Ribonuclease E (RNase E) is a metal-dependent hydrolytic enzyme that cleaves polymeric ribonucleic acid internally and serves as a central element in RNA metabolism of diverse bacteria. The NTD of RNase E (1–529) is highly conserved and harbors the catalytic activity of the enzyme. RNase E forms a tetramer in which the protomers are arranged as a dimer of dimers and accommodate an RNA substrate at the active site formed by the interface of two subunits of the principal dimer unit. The catalytic site is located in a DNase I-like domain, where conserved acidic groups D303 and D346 coordinate the magnesium ions that assist in the hydrolytic attack of single-stranded RNA.

In an effort to structurally characterize the mechanism of 5′ end sensing by RNase E and its interaction with sRNA, the catalytically inactive RNase E (1–529) D303R, D346R was purified and used in co-crystallization trials with sRNA bearing a 5′ monophosphate. The oligoribonucleotide comprises the MicC seed region connected through a tetranucleotide loop with a fragment of the ompD target encompassing the seed complementary sequence and the RNase E cleavage site (Pfeiffer et al., 2009). Crystals of the protein:RNA complex were obtained, and an X-ray diffraction dataset was collected to 3.0 Å resolution. An RNA fragment of 2 to 3 bases could be modeled with a good fit to the density at each of the two independent 5′ sensor domains in the crystallographic asymmetric unit. Given that the 5′ sensor domain is known to bind the 5′ end of RNA substrates, the RNA density was modeled as the 5′ end of MicC. The 5′ monophosphate is bound in the 5′ sensing pocket, and the RNA forms additional contacts with RNase E that were not seen in the previous structure of the “closed” state, where the substrate is bound at the active site. For example, the phosphate backbone is engaged in hydrogen bonding interactions with R373 and R142 in addition to R169 and T170 identified earlier as the core of the 5′ sensing pocket (Callaghan et al., 2005). R141 also contacts the RNA backbone and supports the second base from the 5′ end. Analysis of the crystal structure of E. coli RNase E co-crystallized with the sRNA MicC identified a potential metal ion bound in the RNase H domain not observed in the previous RNase E structures. The coordinating residues at this site are D26, D28, and from the DNase I domain, D338 and R371.

> RHMKRMLINATQQEELRVALVDGQRLYDLDIESPGHEQKKANIYKGKITRIEPSLEAAFVDYGAERHGFLPLKEIAREYFPANYSAHGRPNIKDVLREGQEVIVQIDKEERGNKGAALTTFISLAGSYLVLMPNNPRAGGISRRIEGDDRTELKEALASLELPEGMGLIVRTAGVGKSAEALQWDLSFRLKHWEAIKKAAESRPAPFLIHQESNVIVRAFRDYLRQDIGEILIDNPKVLELARQHIAALGRPDFSSKIKLYTGEIPLFSHYQIESQIESAFQREVRLPSGGSIVIDSTEALTAIRINSARATRGGDIEETAFNTNLEAADEIARQLRLRDLGGLIVIRFIDMTPVRHQRAVENRLREAVRQDRARIQISHISRFGLLEMSRQRLSPSLGESSHHVCPRCSGTGTVRDNESLSLSILRLIEEEALKENTQEVHAIVPVPIASYLLNEKRSAVNAIETRQDGVRCVIVPNDQMETPHYHVLRVRKGEETPTLSYMLPKLHEEAM;> RHMKRMLINATQQEELRVALVDGQRLYDLDIESPGHEQKKANIYKGKITRIEPSLEAAFVDYGAERHGFLPLKEIAREYFPANYSAHGRPNIKDVLREGQEVIVQIDKEERGNKGAALTTFISLAGSYLVLMPNNPRAGGISRRIEGDDRTELKEALASLELPEGMGLIVRTAGVGKSAEALQWDLSFRLKHWEAIKKAAESRPAPFLIHQESNVIVRAFRDYLRQDIGEILIDNPKVLELARQHIAALGRPDFSSKIKLYTGEIPLFSHYQIESQIESAFQREVRLPSGGSIVIDSTEALTAIRINSARATRGGDIEETAFNTNLEAADEIARQLRLRDLGGLIVIRFIDMTPVRHQRAVENRLREAVRQDRARIQISHISRFGLLEMSRQRLSPSLGESSHHVCPRCSGTGTVRDNESLSLSILRLIEEEALKENTQEVHAIVPVPIASYLLNEKRSAVNAIETRQDGVRCVIVPNDQMETPHYHVLRVRKGEETPTLSYMLPKLHEEAMA> NLVQFGVMIEKMTGKS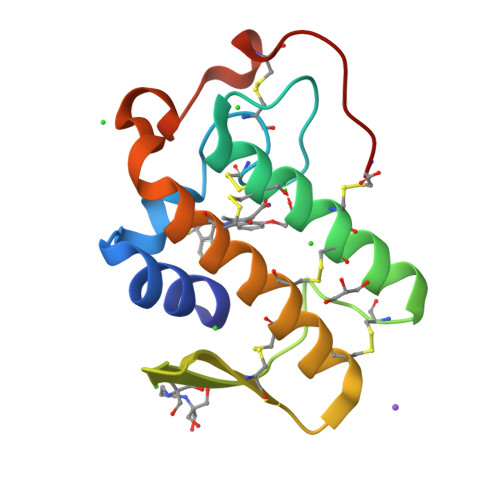ALQYGDYGCYCGIGGSHWPVDQTDWCCHAHDCCYGRLEKLGCEPKLEKYLFSVSERGIFCAGRTTCQRLTCECDKRAALCFRRNLGTYNRKYAHYPNKLCTGPTPPC> MNDIKQLLWNGELNVLVSIDPSFLMKGSPREIAVLRIRVPRETYLVNYMPLIWNKIKSFLSFDPLTDSEKYFWFEHNKTPIPWNYPVGVLFDCLAGKSATFTTSFENQVKDVLTFLRIHLVMGDSLPPTIIPIASSKTQAEKFWFHQWKQVCFILNGSSKAIMSLSVNEARKFWGSVITRNFQDFIEISNKISSSRPRHI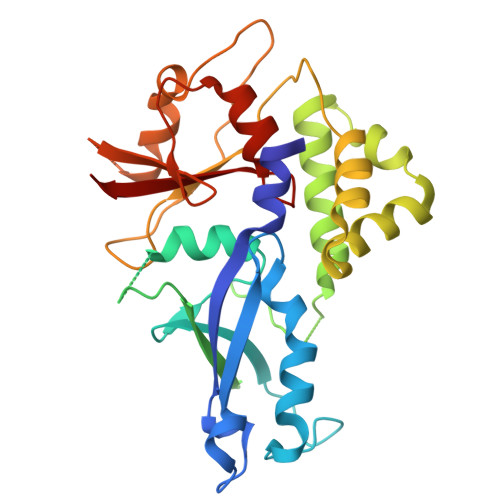PLIIQTSRTSGTFRISQPTISMTGVNPTLKDIEGDILDVKEGINGNDVMVICQGIEIPWHMLLYDLYSKLRSFDGFLYITLVPI>GSGGSIRLADLAQQLDAELHGDGDIVITGVASMQSAQTGHITFMVNPKYREHLGLCQASAVVMTQDDLPFAKSAALVVKNPYLTYARMAQILDTTPQPAQNIAPSAVIDATAKLGNNVSIGANAVIESGVELGDNVIIGAGCFVGKNSKIGAGSRLWANVTIYHEIQIGQNCLIQSGTVVGADGFGYANDRGNWVKIPQIGRVIIGDRVEIGACTTIDRGALDDTIIGNGVIIDNQCQIAHNVVIGDNTAVAGGVIMAGSLKIGRYCMIGGASVINGHMEICDKVTVTGMGMVMRPITEPGVYSSGIPLQPNKVWRKTAALVM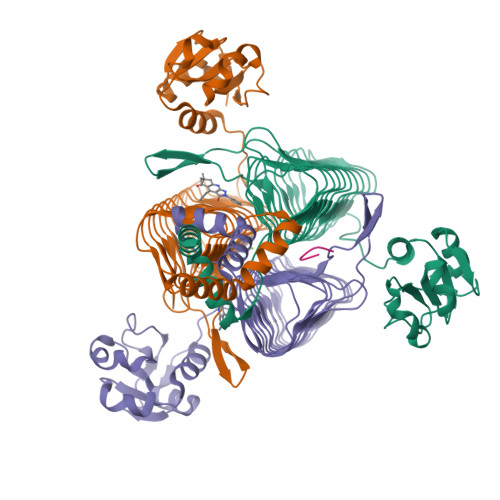NIDDMSKRLKSLERKVNQQD[3x];> TNLYMLPKWDIP>[4x]ATHTLQL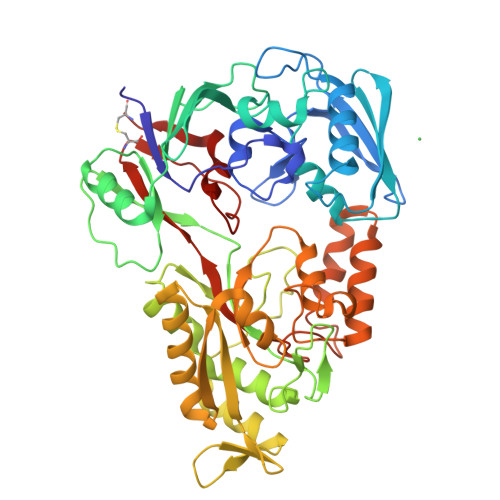AIGDEPTEGFDPMLGWSHGSYLLLHSPLLKQNEDFSWDSLLLSQYQPSDDGKTWLLTLKPDLKFSDGSPLTAKDVAFTYNNAAASGGKVDMGNFLSAEVIDPLNVRIHLKAPQSTFVNVLGSLGIVSADKYNAKTYAQKPIGAGPYRLVSFQPGQQMIVEANPYYAGNKNDFDKLIFVFLDEDSAFAAAQSGQLGVVRIPPSMAVGSVNNMKLWVRPSVENRGIVFPTTPAGKKDAHGYPIGNDVTADVAIRRAINYAINRQLLADQIMEGHAIPAYTGVQGLPWNNPDSAIKDGDIDKAKQILEQAGWQLNSQGTREKNGLPAKITLWYTSGDTTRRDLAQALRSMLKPIGIDVDLKSGSWETVERNMHANPTLFGWGSLDPMELYHHYSSNAAGVEYYNPGYYKNPMVDKHLQQALDAPTWQQAVPFWQQVDWDGTTGAGIRGDAAWAWLLNIQHTYLANNCVDLGKGTPEIHGSWSLLNSIDSWKWTCQ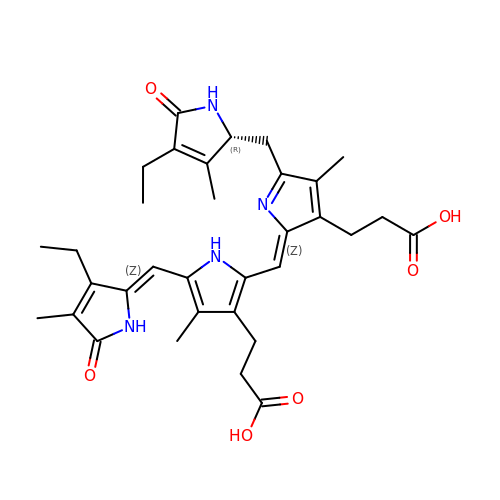DiCys-(15,16)-Dihydrobiliverdin | C33 H40 N4 O6 | MZFCOERRVCGRTL-ZTYGKHTCSA-N>[2x]MKTIIINGVQFNTDEDTTILKFARDNNIDISALCFLNNCNNDINKCEICTVEVEGTGLVTACDTLIEDGMIINTNSDAVNEKIKSRISQLLDIHEFKCGPCNRRENCEFLKLVIKYKARASKPFLPKDKTEYVDERSKSLTVDRTKCLLCGRCVNACGKNTETYAMKFLNKNGKTIIGAEDEKCFDDTNCLLCGQCIIACPVAALSEKSHMDRVKNALNAPEKHVIVAMAPSVRASIGELFNMGFGVDVTGKIYTALRQLGFDKIFDINFGADMTIMEEATELVQAIENNGPFPMFTSCCPGWVRQAENYYPELLNNLSSAKSPQQIFGTASKTYYPSISGLDPKN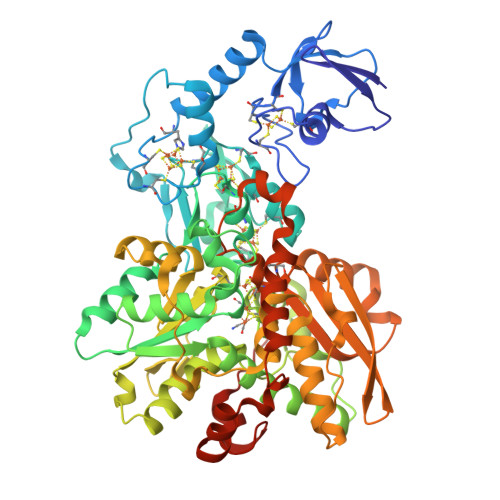VFTVTVMPCTSKKFEADRPQMEKDGLRDIDAVITTRELAKMIKDAKIPFAKLEDSEADPAMGEYSGAGAIFGATGGVMEAALRSAKDFAENAELEDIEYKQVRGLNGIKEAEVEINNNKYNVAVINGASNLFKFMKSGMINEKQYHFIEVMACHGGCVNGGGQPHVNPKDLEKVDIKKVRASVLYNQDEHLSKRKSHENTALVKMYQNYFGKPGEGRAHEILHFKYKKSAWSHPQFEK6-(4-chloro-2-fluoro-3-phenoxybenzyl)pyridazin-3(2H)-one | C17 H12 Cl F N2 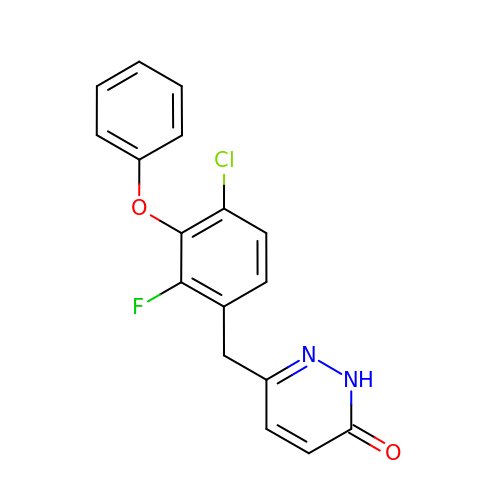O2 | NOVPOXGMADEKPP-UHFFFAOYSA-N Ornithine carbamoyltransferases (OTCs) are involved in the arginine deiminase (ADI) pathway and in arginine biosynthesis. Two OTCs in a pair are named catalytic OTC (cOTC) and anabolic OTC (aOTC). Structural and biochemical analyses were employed to investigate the CP cooperativity and unidirectional function of two sequentially similar OTCs (32.4% identity) named Ps_cOTC and Ps_aOTC from Psychrobacter sp. PAMC 21119. Here, we determined the Ps_cOTC and Ps_aOTC structures from the psychrophilic bacteria Psychrobacter sp. PAMC 21119 at 2.6 and 2.2 Å and compared them in respect to the substrate preferences for kinetic processes and cooperativity.

In contrast, aOTC catalyzes the biosynthesis of citrulline from CP and ornithine in vivo and is thus involved in arginine biosynthesis. Moreover, we determined the crystal structure of Ps_aOTC at a 2.2 Å resolution. Most of the amino acids were built, except for the SMG loop region (nine amino acids) between S8 and H10 because of ambiguous electron density. In detail, His131 from H6; Asn162 and Met163 from H7; the Cys259, Leu260, and Ala262 from the HCLP loop; and Arg55 from H3 are the main residues creating the potential binding cleft for the CP and ORN of Ps_aOTC. These residues are highly conserved among OTCs indicating that Ps_aOTC may have the catalytic characteristics of aOTCs. Three identical Ps_aOTC monomers are built from a cyclic homotrimer, which shows a similar quaternary structure as Ps_cOTC. In the Ps_aOTC structure, the 80s loop (81–LGRGEP–86) is leaning against the H5 of the B chain starting from the sharp turn of P86. Conversely, Ps_aOTC forms a potential binding cavity for CP. The clear CP and ORN binding sites provided by the lack of closed residues from the 80s loop in the Ps_aOTC probably allow the CP molecule to slip into the binding site. Ps_aOTC also exhibited thermal stability in concert with elevated CP concentrations but with a hyperbolic pattern.

>[2x]GSHMSLRHFLTLSDLTKQELENLIKRASELRKMQHAGEIYQPFVGRTLGMIFEKSSTRTRISFETGMGQFGGNAIFLSPNDTQLGRGEPLEDSARVISSMVDIIMIRTFGHEKVETFAEYSSVPIINALTDDYHPCQLLADMQTYYEHRGSIENKIVTWVGDGNNMCSSFMQAANQFGFELRVAAPYGFEPDPKLMERFSHCVSLVENVQDAAKDANLIVTDVWASMGQESEQNTRARRFAPYQVTPSLLDKADPEVVFMHCLPAHRGEEISHDMLNDPRSVVWDEAENRLHAQKALMEFLLKDKIKI> MAQINVIGQNGGRTIELPLPEVNSGVLHEVVTWQLASRRRGTASTRTRAQVSKTGRKMY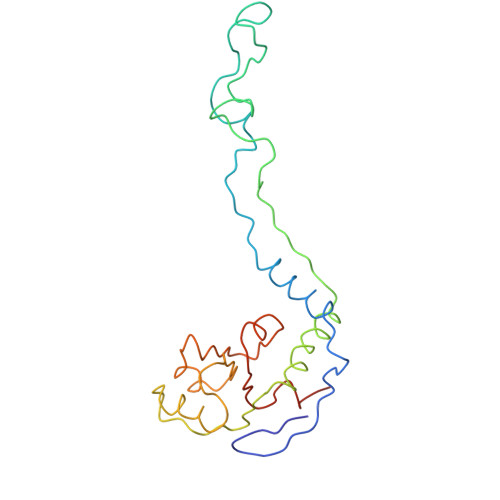GQKGTGNARHGDRSVPTFVGGGVAFGPKPRSYDYTLPRQVRQLGLAMAIASRQEGGKLVAVDGFDIADAKTKNFISWAKQNGLDGTEKVLLVTDDENTRRAARNVSWVSVLPVAGVNVYDILRHDRLVIDAAALEIVEEEAGEEQQ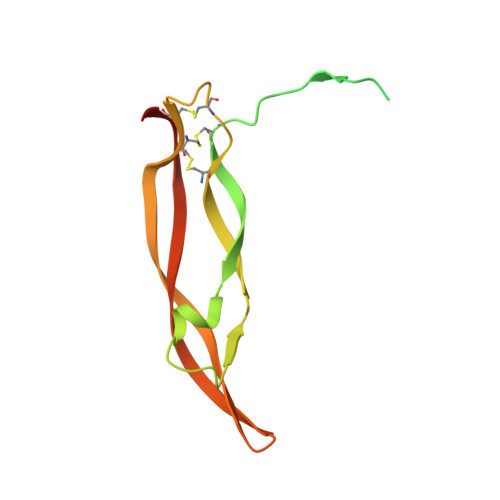> EGDPIPEELYEMLSDHSIRSFDDLQRLLHGDPGEEDGAELDLNMTRSHSGGELESLARGRRSLGSLTIAEPAMIAECKTRTEVFEISRRLIDRTNANFLVWPPCVEVQRCSGCCNNRNVQCRPTQVQLRPVQVRKIEIVRKKPIFKKATVTLEDHLACKCETVAAHHHHHHH> ADTIVAVELDTYPNTDIGDPSYPHIGIDIKSVRSKKTAKWNMQDGKVGTAHIIYNSVDKRLSAVVSY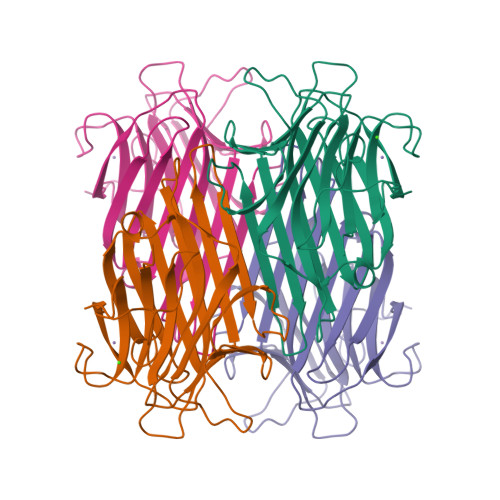PNADATSVSYDVDLNDVLPEWVRVGLSASTGLYKETNTILSWSFTSKLKSNSTHQTDALHFMFNQFSKDQKDLILQGDATTGTDGNLELTRVSSNGSPEGSSVGRALFYAPVHIWESSATVSAFEATFAFLIKSPDSHPADGIAFFISNIDSSIPSGSTGRLLGLFPDAN DODECANESULFONATE 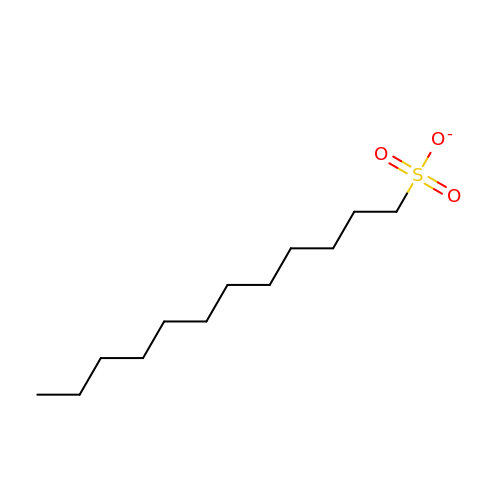ION | C12 H25 O3 S | LDMOEFOXLIZJOW-UHFFFAOYSA-M>[2x]MALVYDAEFVGSEREFEEERETFLKGVKAYDGVLATRYLMERSSSAKNDEELLELHQNFILLTGSYACSIDPTEDRYQNVIVRGVNFDERVQRLSTGGSPARYAIVYRRGWRAIAKALDIDEEDVPAIEVRAVKRNPLQPALYRILVRYGRVDLMPVTVDEVPPEMAGEFERLIERYDVPIDEKEERILEILRENPWTPHDEIARRLGLSVSEVEGEKDPESSGIYSLWSRVVVNIEYDERTAKRHVKRRDRLLEELYEHLEELSERYLRHPLTRRWIVEHKRDIMRRYLEQRIVECALKLQDRYGIREDVALCLARAFDGSISMIATTPYRTLKDVCPDLTLEEAKSVNRTLATLIDEHGLSPDAADELIEHFESIAGILATDLEEIERMYEEGRLSEEAYRAAVEIQLAELTKKEGVGRKT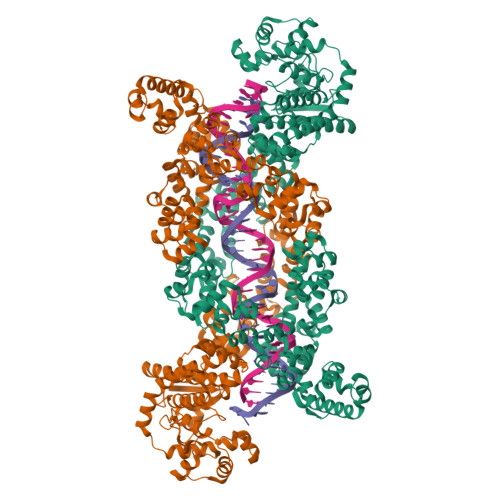AERLLRAFGNPERVKQLAREFEIEKLASVEGVGERVLRSLVPGYASLISIRGIDRERAERLLKKYGGYSKVREAGVEELREDGLTDAQIRELKGLKTLESIVGDLEKADELKRKYGSASAVRRLPVEELRELGFSDDEIAEIKGIPKKLREAFDLETAAELYERYGSLKEIGRRLSYDDLLELGATPKAAAEIKGPEFKFLLNIEGVGPKLAERILEAVDYDLERLASLNPEELAEKVEGLGEELAERVVYAARERVESRRKSGRQERSEEEWKEWLERKVGEGRARRLIEYFGSAGEVGKLVENAEVSKLLEVPGIGDEAVARLVPGYKTLRDAGLTPAEAERVLKRYGSVSKVQEGATPDELRELGLGDAKIARILGLRSLVNARLDVDTAYELARRYGSVSAVRAAPVAELRELGLSDRAIARIAGIP> MEKSVSVILLAGGQGKRMKMSMPKQYIPLLGQPIALYSFFTFSRMPEVKEIVVVCDPFFRDIFEEYEESIDVDLRFAIPGKERQDSVYSGLQEIDVNSELVCIHDSARPLVNTEDVEKVLKDGSAVGAAVLGVPAKATIKEVNSDSLVVKTLDRKTL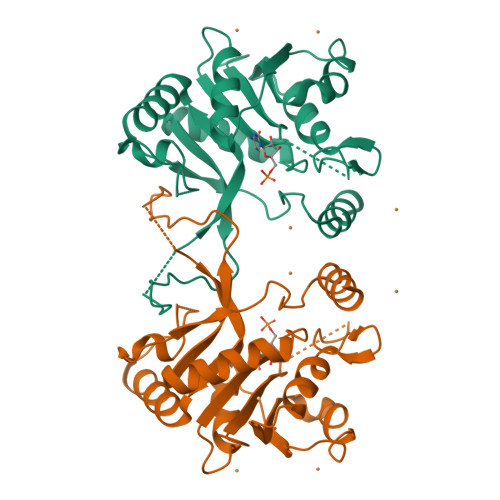WEMQTPQVIKPELLKKGFELVKSEGLEVTDDVSIVEYLKHPVYVSQGSYTNIKVTTPDDLLLAERILSEDS> AQYEDGKQYTTLEKPVAGAPQVLEFFSFFCPHAYQFEEVLHISDNVKKKLPEGVKMTKYHVNFMGGDLGKDLTQAWAVAMALGVEDKVTVPLFEGVQKTQTIRSASDIRDVFINAGIKGEEYDAAWNSFVVKSLVAQQEKAAADVQLRGVPAMFVNGKYQLNPQGMDTSN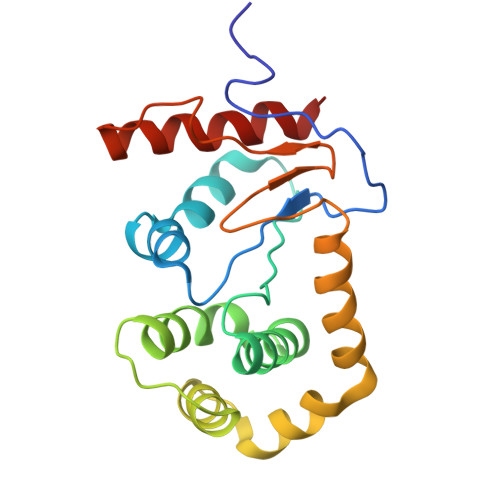MDVFVQQYADTVKYLSEKK>[3x]MRMSDGAAPKANGSEASGQDLVPAAVEQAVPIQPVAGAALAAPAAGQINQIDPWIFQNFVQCPLGEFSISPRNTPGEILFDLALGPGLNPYLAHLSAMYTGWVGNMEVQLVLAGNAFTAGKVVVALVPPYFPKGSLTTAQITCFPHVMCDVRTLEPIQLPLLDVRRVLWHATQDQEESMRLVCMLYTPLRTNSPGDESFVVSGRLLSKPAADFNFVYLTPPIERTIYRMVDLPVIQPRLCTHARWPAPVYGLLVDPSLPSNPQWQNGRVHVDGTLLGTTPISGSWVSCFAAEAAYEFQSGTGEVATFTLIEQDGSAYVPGD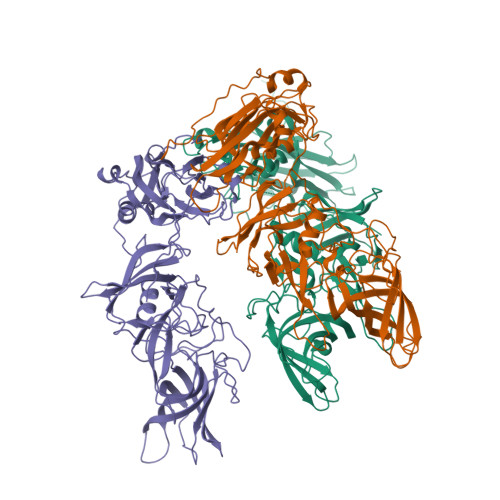RAAPLGYPDFSGQLEIEVQTETTKTGDKLKVTTFEMILGPTTNADQAPYQGRVFASVTAAASLDLVDGRVRAVPRSIYGFQDTIPEYNDGLLVPLAPPIGPFLPGEVLLRFRTYMRQIDTADAAAEAIDCALPQEFVSWFASNAFTVQSEALLLRYRNTLTGQLLFECKLYNEGYIALSYSGSGPLTFPTDGIFEVVSWVPRLYQLASVGSLATGRMLKQ The starting point of the engineering efforts reported here is a Kemp eliminase we previously obtained through minimalist design on a β-lactamase background. Our design took advantage of the conformational flexibility of an ancestral β-lactamase scaffold to produce both a suitable cavity and a catalytic base within it through a single mutation, while a second mutation enhanced relevant interactions at the de novo active site. Kemp elimination is a straightforward proton–abstraction reaction that can be performed by a simple molecular machinery consisting, at the bare minimum, of a catalytic base. FuncLib does not per se predict mutations that enhance catalysis, but rather suggests variants with multiple mutations that generate stabilizing interacting networks at the active site, thus focusing the search to safe regions of the sequence space.

Finally, we have used X-ray crystallography to determine the 3D-structures of the catalytically optimized GNCA4-2, GNCA4-12 and GNCA4-19 variants, the first of which has a transition state analogue bound at the de novo active site. These particular structures were chosen as they are all highly active variants, in terms of the measured rates within the available substrate concentration range, with improved catalytic parameters over GNCA4-WT. The protein backbones of these new structures are essentially superimposable with that of the background GNCA4-WT variant and, therefore, the observed enhancement of catalysis is likely linked to small rearrangements in the de novo active site. Here, our crystal structures illustrate that significant gains in activity can be achieved without the need for corresponding significant active site rearrangement. To assess this, we also performed EVB simulations on the variants for which crystal structures were available: GNCA-2, GNCA-12 and GNCA-19. For these variants, the calculated values fall to within 1.3 kcal mol–1 of the experimental values, and can deviate by up to 2.2 kcal mol–1 from the values calculated from the FuncLib predicted structures.

> AAALSEQLAELEKRSGGRLGVAVLDTATGRRFGYRGDERFPMCSTFKALLAAAVLARVDQGKENLDRRITYGKEDLVDYSPVTEKHVGDGMTVAELCEAAITYSDNTAANLLLEALGGPAALTAFLRSIGDNVTRLDRWEPELNTAAPGDPRDTTTPAAMAATLRTLLLGDVLSPASRQQLVDWLIANKTGDKRLRAGLPADDRVGDKTGTGEHGTTNDIAVVWPPNHAPIFIAVYLTESQVDADARDAVIAEVARLIVAAWHHHHHH>[2x]MASWSHPQFEKMGMLEARELLCERDERTLFSGLSFTLNAGEWVQITGSNGAGKTTLLRLLTGLSRPDAGEVLWQGQPLHQVRDSYHQNLLWIGHQPGIKTRLTALENLHFYHRDGDTAQCLEALAQAGLAGFEDIPVNQLSAGQQRRVALARLWLTRATLWILDEPFTAIDVNGVDRLTQRMAQHTEQGGIVILTTHQPLNVAES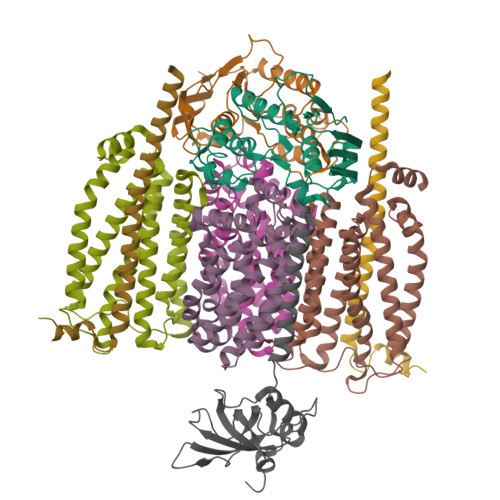KIRRISLTQTRAA;>MMFWRIFRLELRVAFRHSAEIANPLWFFLIVITLFPLSIGPEPQLLARIAPGIIWVAALLSSLLALERLFRDDLQDGSLEQLMLLPLPLPAVVLAKVMAHWMVTGLPLLILSPLVAMLLGMDVYGWQVMALTLLLGTPTLGFLGAPGVALTVGLKRGGVLLSILVLPLTIPLLIFATAAMDAASMHLPVDGYLAILGALLAGTATLSPFATAAALRISIQ[2x];>MWKTLHQLAIPPRLYQICGWFIPWLAIASVVVLTVGWIWGFGFAPADYQQGNSYRIIYLHVPAAIWSMGIYASMAVAAFIGLVWQMKMANLAVAAMAPIGAVFTFIALVTGSAWGKPMWGTWWVWDARLTSELVLLFLYVGVIALWHAFDDRRLAGRAAGILVLIGVVNLPIIHYSVEWWNTLHQGSTRMQQSIDPAMRSPLRWSIFGFLLLSATLTLMRMRNLILLMEKRRPWVSELILKRGRK[2x];>MTPAFASWNEFFAMGGYAFFVWLAVVMTVIPLVVLVVHSVMQHRAILRGVAQQRAREARLRAAQQQEAA[2x];> MNIRRKNRLWIACAVLAGLALTIGLVLYALRSNIDLFYTPGEILYGKRETQQMPEVGQRLRVGGMVMPGSVQRDPNSLKVTFTIYDAEGSVDVSYEGILPDLFREGQGVVVQGELEKGNHILAKEVLAKHDENYTPPEVEKAMEANHRRPASVYKDPAS N-[(3-methoxyphenyl)methyl]-5H-[1]benzopyrano[3,4-c]pyridine-8-carboxamide | C21 H18 N2 O3 | 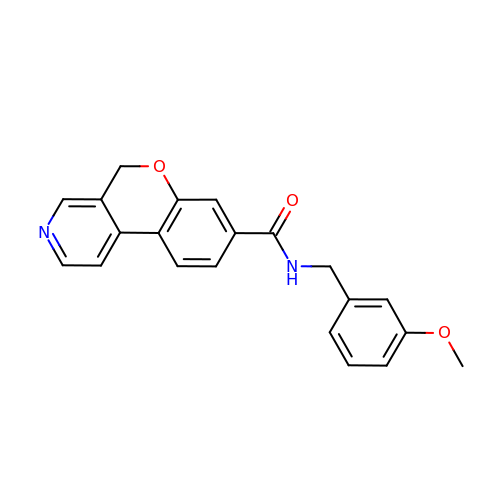SIKMVWPMDNIKAY-UHFFFAOYSA-N> LHEAKEREELRREVRELIEEGKTAEEIAEILGLSVDEIKELIGRREVRELIEEGKTAEEIAEILGLSVDEIKELIGRREVRELIEEGKTAEEIAEILGLSVDEIKELIGRREVRELIEEGKTAEEIAEILGLSVDEIKELIGRREVR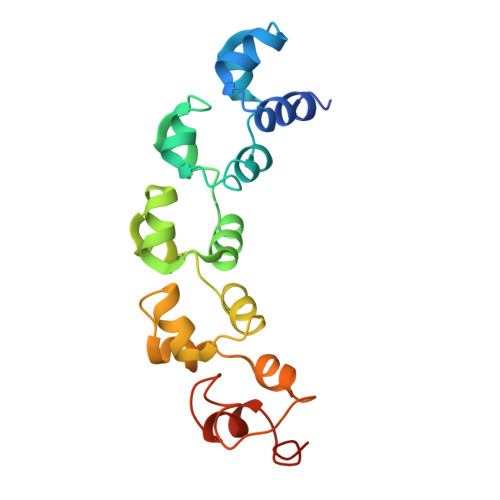ELIEEGKTAEEIAEILGLSVDEIKELIGEEEIKKIEEK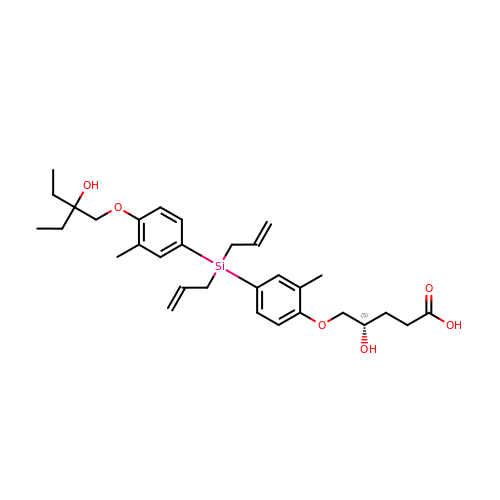(4~{S})-5-[4-[[4-(2-ethyl-2-oxidanyl-butoxy)-3-methyl-phenyl]-bis(prop-2-enyl)silyl]-2-methyl-phenoxy]-4-oxidanyl-pentanoic acid | C31 H44 O6 Si | ACVDDFOGQPPGOI-RUZDIDTESA-N> NLYQFKNMIQCTVPSRSWADFADYGCYCGKGGSGTPVDDLDRCCQTHDNCYNEAENISGCRPYFKTYSYECTQGTLTCKGDNNACAASVCDCDRLAAICFAGAPYN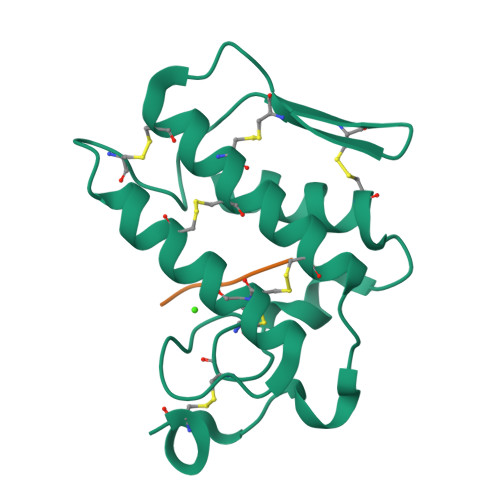DANYNIDLKARCN;> VAFRS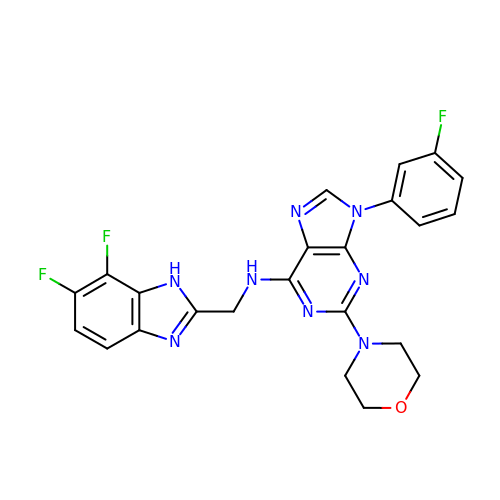~{N}-[[6,7-bis(fluoranyl)-1~{H}-benzimidazol-2-yl]methyl]-9-(3-fluorophenyl)-2-morpholin-4-yl-purin-6-amine | C23 H19 F3 N8 O | CEBMEQPREMCWOL-UHFFFAOYSA-N> HPYYLRSFLVVLKTVLENEDDMLLFDEQEKGIVTKFYQLSATGQKLYVRLFQRKLSWIKMTKLEYEEIALDLTPVIEELTNAGFLQTESELQELSEVLELLSAPELKSLAKTFHLVNPNGQKQQLVDAFLKLAKQRSVCTWGKNKPGIGAVILKRAKALAGQSVRICKGPRAVFSRILLLFSLTDSMEDEDAACGGQGQLSTVLLVNLGRMEFPSYTINRKTHIFQDRDDLIRYAAATHMLSDISSAMANGNWEEAKELAQCAKRDWNRLKNHPSLRCHEDLPLFLRCFTVGWIYTRILSRFVEILQRLHMYEEAVRELESLLSQRIYCPDSRGRWWDRLALNLHQHLKRLEPTIKCITEGLADPEVRTGHRLSLYQRAVRLRESPSCKKFKHLFQQLPEMAVQDVKHVTITGRLCPQRGMCKSVFVMEAGEAADPTTVLCSVEELALAHYRRSGFDQGIHGEGSTFSTLYGLLLWDIIFMDGIPDVFRNACQAFPLDLCTDSFFTSRRPALEARLQLIHDAPEESLRAWVAATWHEQEGRVASLVSWDRFTSLQQAQDLVSCLGGPVLSGVCRHLAADFRHCRGGLPDLVVWNSQSRHFKLVEVKGPNDRLSHKQMIWLAELQKLGAEVEVCHVV

FAN1 (FANCD2-FANCI-associated nuclease 1) is a DNA structure-dependent nuclease ubiquitously expressed in the central nervous system and peripheral tissues that plays a role in resolving interstrand crosslinks at replication forks. It possesses both 5′ flap endonuclease and 5′-3′ exonuclease activities, allowing it to process DNA structures that arise during replication stress and repair pathways. FAN1 comprises a DNA-binding SAF-A/B, Acinus and PIAS (SAP) domain, a tetratricopeptide repeat (TPR) domain that mediates dimerization and protein-protein interactions, a virus-type replication-repair nuclease module (VRR) containing the catalytic site, and an unstructured N-terminal region5. PCNA is a homotrimeric ring-shaped DNA clamp that encircles double-stranded DNA after being loaded by replication factor C (RFC).

For the structural studies, we chose the canonical double flap DNA substrate over a CAG extrahelical extrusion containing DNA, because the 5′ phosphate of the post-nick strand is essential for tight coordination of the DNA to the NUC domain. This reduces the flexibility of this domain, resulting in more rigid particles and thereby enabling higher resolution structures. Indeed, the structural analysis revealed side-chain densities for the amino acids R706, H742, R952, R955, K986 in the NUC domain coordinating the 5′-phosphate. However, despite the high-resolution of the SAP domain, the flexibility of the dimerization loop prevented us from resolving R507. We solved the cryo-EM structure of the full-length FAN1–DNA complex and found that the flexibility of the 510-519 loop hindered our ability to again resolve the R507 residue. The unresolved loop region of FAN1 in the FAN1–DNA complex (middle). Additional structural comparisons between the FAN1–DNA and FAN1–PCNA–DNA complexes revealed that the angle of the 5′ flap double-stranded DNA substrate remains fixed at 68°, and no significant conformational changes were observed in FAN1 between the two complexes. F Overall structural comparison between FAN1–PCNA–DNA (gray) and FAN1–DNA (black) complexes reveals no significant conformational changes in FAN1 upon binding to PCNA.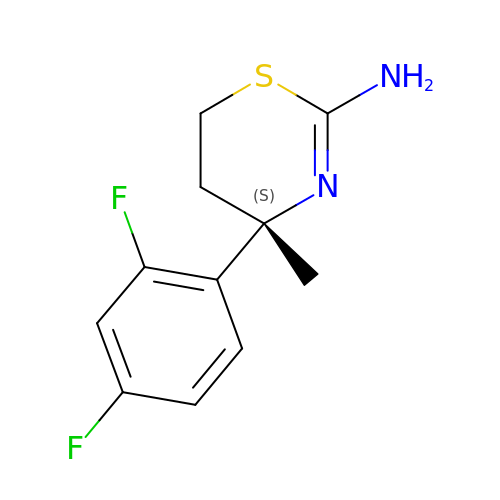(4S)-4-(2,4-difluorophenyl)-4-methyl-5,6-dihydro-4H-1,3-thiazin-2-amine | C11 H12 F2 N2 S | JRYNZJXSUKTLGF-NSHDSACASA-N> MGSSHHHHHHSSENLYFQGHMKAEVSQQRSLLTLSEVDAELARIAHRGKNLAEQKRLDELTAQRGEVNDRLAALGIALEDLDAQVAKYESEIDSVRQREDRDRALLEGGSVGAKQVTEIQHELETLQRRQASLEEQLLEVMERREELMAERSEELRRVDELQTELTEAQQARDAALVELDQARHQCATRRDALVNAIDDQLVELYEKQR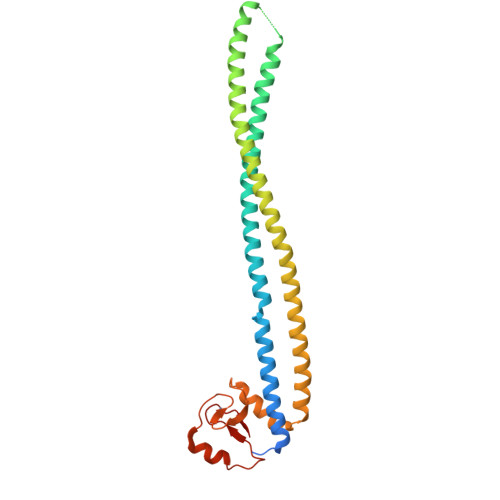ARGGAGAGPLQGRRCGACRIEIDRGEIARITAAADDDVVRCPECGAILLRVKQ>[2x]MSQVGGRGDRCTQEVQGLVHGAGDLSASLAENSPTMSQNGYFEDSSYYKCDTDDTFEAREEILGDEAFDTANSSIVSGESIRFFVNVNLEMQATNTENEATSGGCVLLHTSRKYLKLKNFKEEIRAHRDLDGFLAQASIVLNETATSLDNVLRTMLRRFARDPDNNEPNCNLDLLMAMLFTDAGAPMRGKVHLLSDTIQGVTATVTGVRYQQSWLCIICTMKALQKRHVCISRLVRPQNWGENSCEVRFVILVLAPPKMKSTKTAMEVARTFATMFSDIAFRQKLLETRTEEEFKEALVHQRQLLTMVSHGPVAPRTKERSTVSLPAHRHPEPPKCKDFVPFGKGIREDIARRFPLYPLDFTDGIIGKNKAVGKYITTTLFLYFACLLPTIAFGSLNDENTDGAIDVQKTIAGQSIGGLLYALFSGQPLVILLTTAPLALYIQVIRVICDDYDLDFNSFYAWTGLWNSFFLALYAFFNLSLVMSLFKRSTEEIIALFISITFVLDAVKGTVKIFWKYYYGHYLDDYHTKRTSSLVSLSGLGASLNASLHTALNASFLASPTELPSATHSGQATAVLSLLIMLGTLWLGYTLYQFKKSPYLHPCVREILSDCALPIAVLAFSLISSHGFREIEMSKFRYNPSESPFAMAQIQSLSLRAVSGAMGLGFLLSMLFFIEQNLVAALVNAPENRLVKGTAYHWDLLLLAIINTGLSLFGLPWIHAAYPHSPLHVRALALVEERVENGHIYDTIVNVKETRLTSLGASVLVGLSLLLLPVPLQWIPKPVLYGLFLYIALTSLDGNQLVQRVALLLKEQTAYPPTHYIRRVPQRKIHYFTGLQVLQLLLLCAFGMSSLPYMKMIFPLIMIAMIPIRYILLPRIIEAKYLDVMDAEHRP

BTR1 (SLC4A11) is a NH3 stimulated H+ (OH-) transporter belonging to the SLC4 family. Dysfunction of BTR1 leads to diseases such as congenital hereditary endothelial dystrophy (CHED) and Fuchs endothelial corneal dystrophy (FECD). BTR1 shares a similar membrane topology with other SLC4 family members, with its substrate binding sites located in the central cavity between the gate and core domains. The TMD contains a core domain (comprising TMs 1–4 and 8–11) and a gate domain (comprising TMs 5–7 and 12–14), resembling the arrangement of UraA25.

Loss of function of BTR1 caused by the R125H mutation has been widely reported. Given that the binding of PIP2 is pH sensitive and histidine is less positively charged than arginine under physiological pH conditions, we presume that the pathogenesis of R125H mutation can be attributed to the charge alteration of the L site which in turn adversely affects the binding of PIP2, ultimately leading to the impaired transport activity of BTR1. To further explore how PIP2 participates in the complete substrate transport process of BTR1 and prove the connection between PIP2 and pH sensing, we attempted to solve the structures of BTR1 with the R125H mutation or wild-type BTR1 prepared under acidic pH, which may both disrupt the interaction between BTR1 and PIP2, and succeed in achieving resolutions of 2.96 Å and 2.94 Å, respectively. Intriguingly, two structures are nearly indistinguishable in conformation (RMSD = 0.250 Å), and both lack the densities of PIP2. Compared with the structures of BTR1 in the outward-facing state, the distinct features of the non-PIP2 binding BTR1 structures involve that the NTD has undergone a significant twist, as well as an apparent conformational change has taken place in the TMD. Analysis of the TMDs using HOLE2 shows that the substrate binding sites of BTR1 in these two states are accessible from the intracellular side, suggesting their inward-facing conformation. The structural alignment of the TMDs of BTR1OF/APO state and BTR1IF/R125H state by the gate domains shows that, during the conformation transition process from the outward-facing state to the inward-facing state, the gate domains remain relatively unchanged (RMSD = 1.678 Å), but an obvious displacement has occurred in the core domains (RMSD = 3.784 Å). The core domain of BTR1OF/APO state needs to go through a 12.38° rotation and a 7.4 Å shift towards the gate domain to reach the position of core domain of BTR1IF/R125H state. In comparison with the alteration of the TMD caused by the disruption of the interaction between PIP2 and BTR1 during the state transition process, the conformation of the NTD changes even more significantly. The NTD has undergone a 175.9 ° deflection and a 24.9 Å position shift from BTR1OF/APO state to BTR1IF/R125H state conformation.Here we show that Bdellovibrio bacteriovorus utilizes a small ankyrin repeat protein, Bd3460, to protect itself from endopeptidase activities during entry of prey. We demonstrate that endopeptidase complexation by Bd3460 prevents cell wall decrosslinking, and that both the Bd0816 and Bd3459 targets bind this self-protection protein via a common epitope. Previously, we assigned prey cell rounding to the action of two secreted Bdellovibrio peptidoglycan DD-endopeptidases, Bd0816 and Bd3459, that act to modify the invaded cell wall via hydrolysis of the structural 3-4 peptide crosslinks6. In summary, we conclude that we have identified and characterized the first ever self-protection protein encoded by predatory bacteria—ankyrin repeat protein Bd3460 from Bdellovibrio inhibits the prey wall decrosslinking enzymes Bd3459/Bd0816 and in doing so protects the predator from the shape transition that this catalyses in prey.

The use by B. bacteriovorus (and related periplasmic predators) of multiple DD-endopeptidases to decrosslink prey wall, and our observation of specific neutralization of Bd3459 by Bd3460 raised the question as to whether a similar mechanism is used to protect against Bd0816. Bd0816 expression was toxic but was circumvented by mutating the active site Serine residue to Alanine (S58A). The resulting 2.48 Å structure of the Bd0816:Bd3460 complex reveals a conserved mode of binding between the ARP self-protection protein and both predatory DD-endopeptidase targets. Bd0816 is largely structurally equivalent to Bd3459, with a few small differences in surface-exposed loops (loops involved in Bd0816 oligomerization). It is striking that we observe a trimeric form of Bd0816 (burying 1,041 A2 of surface area per monomer, on the borderline for statistically significant oligomers). In-vitro characterization of the Bd0816:Bd3460 complex suggests the 1:1 heterodimer likely represents the dominant form in solution. Comparison of the residues involved in both complexes illustrates that the endopeptidase:self-protection protein interface is conserved, and is likely to be representative of protection mechanisms in related predators.

>[6x]MVYVNSVCHMKAAATAGKVEGEGDMQKKFPLAAISKVITTLWAIEKLGVDYRHKTVLHLTPTANGSMDLHVEGSRDPIFGRNLSYFLISELNRMKVTKIENLTFDENFLLDWLAEESPRIGGVTPRYETIEQQAEAVIKNLKESFSTAINRAMYSKLRERATKAKVFMLEKPTIEVRNISFLPKNNYKKDKYTGSVVLQSAPLRTILKRMNNQSNNYIADNLYWNLGGTAAFNAFAAATLKADQNQIVFHNGSGNNEGTTAKPIYNEATCETMIKTLYTLNKSLEAKGYKLSDVLSVANKDSDSTIDNFGGNAAGSMIAKTGTVNKAKTLAGSISTKEGEFYFAILLHTDMDQSSSDRGVASQMIKNKISQLINKRSGPKEIQYTEILALPFDQNSYLTEA;>KSSKALNEAAEQGDLAKVKNLVQKNKIDLNAQDETGMTPLMNAAMGGNLDIVKFLLSKKVNLELKNNGGETALAFAVTNDAYDVAEELIKAGANVDIIVAGDEGDTLFMRAAQNNKKTAESILAKNKSLINKANTLGETALFAVARYGTPADIDFLIKKGADLKLKNKKGQTALDVAKEASNQDTAKALSKKK[6x]(2~{R},3~{S},4~{R},5~{R},6~{S})-2-(hydroxymethyl)-6-(2-naphthalen-2-yl-1~{H}-imidazol-4-yl)oxane-3,4,5-triol 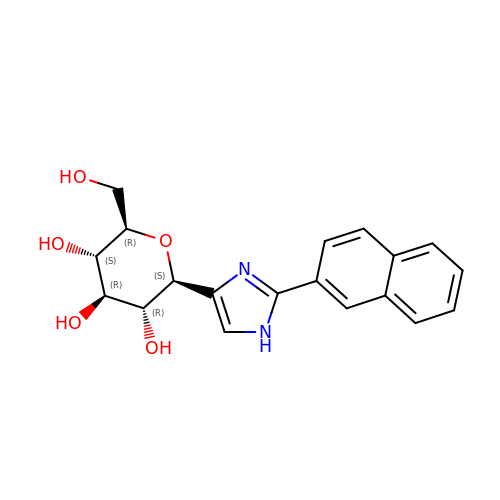| C19 H20 N2 O5 | VRUXFQSZTNCMBM-SFFUCWETSA-N> PDCGVICENGKCVVKENGSNCRHYNIYEPAPDVKTTEINVIVSGDEQGIITKKLQDFCMNPNNENGTNNQIWKCYYKDEKEDKCKVETKSGNSTYKEKITSFDEFFDFWVRKLLIDTIKWETELTYCINNTTNADCNNECNKNCVCFDKWVKQKEKEWKNIMDLFTNKHDIPKKYYLNINDLFNSFFFQVIYKFNEGEAKWNKLKENLKKKTESSKKNKGTKDSEAAIKVLFDHLKETATICKDNNTNEAC;> LQRLHMLQISYFRDPYHVWYQGNASLGGHLTHVLEGPDTNTTIIQLQPLQEPESWARTQSGLQSYLLQFHGLVRLVHQERTLA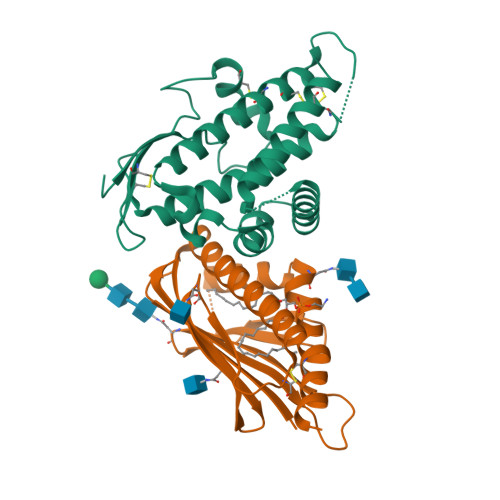FPLTIRCFLGCELPPEGSRAHVFFEVAVNGSSFVSFRPERALWQADTQVTSGVVTFTLQQLNAYNRTRYELREFLEDTCVQYVQKHIS> GQQPDAKNILERTAEAFRKAGGVKLAFTVNEQQGSYAGVLYLEGEKFVVETEGMKTW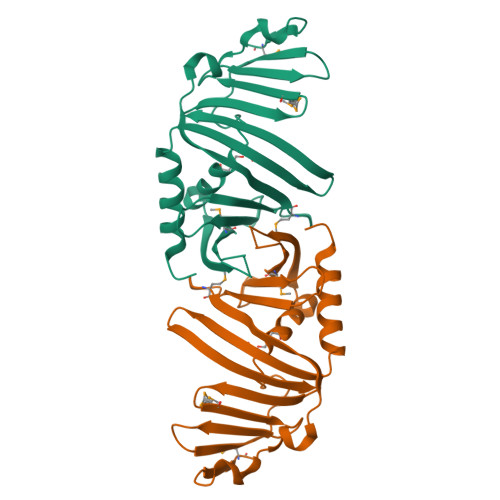FDGHTQWSYVASADEVNVSEPTQEELQTLNPYAWLSLYKQGYRLKLSSVGGKQDKSVYYITMTAADKRKDPESVYLFVTKDTYRLHQVDLAPRGSKYMTTILIDSYQTGQSYPDSFFVFDKKAYPTAEVIDMR> CGCCCGGAUAGCUCAGUCGGUAGAGCAGCGGCU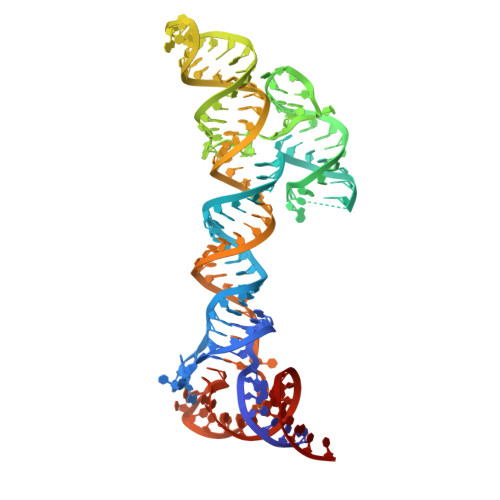AAAACAGCUCUGGGGUUGUACCCACCCCAGAGGCCCACGUGGCGGCUAGUACUCCGGUAUUGCGGUACCCUUGUACGCCUGUUUUAGCCGCGGGUCCAGGGUUCAAGUCCCUGUUCGGGCGCCA>[2x]LLAGASSQRSVARMDGDVIIGALFSVHHQPPAEKVPERKCGEIREQYGIQRVEAMFHTLDKINADPVLLPNITLGSEIRDSCWHSSVALEQSIEFIRDSLISIRDEKDGINRCLPDGQSLPPGRTKKPIAGVIGPGSS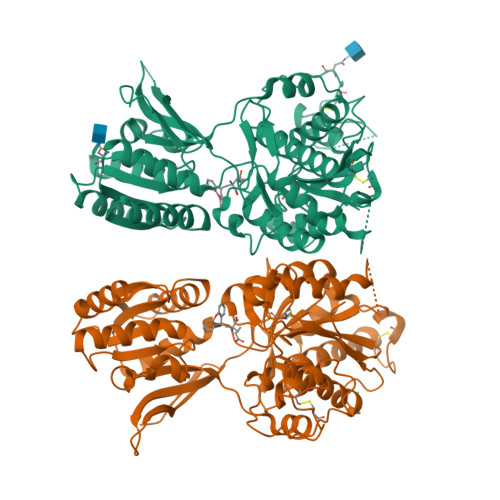SVAIQVQNLLQLFDIPQIAYSATSIDLSDKTLYKYFLRVVPSDTLQARAMLDIVKRYNWTYVSAVHTEGNYGESGMDAFKELAAQEGLSIAHSDKIYSNAGEKSFDRLLRKLRERLPKARVVVCFCEGMTVRGLLSAMRRLGVVGEFSLIGSDGWADRDEVIEGYEVEANGGITIKLQSPEVRSFDDYFLKLRLDTNTRNPWFPEFWQHRFQCRLPGHLLENPNFKRICTGNESLEENYVQDSKMGFVINAIYAMAHGLQNMHHALCPGHVGLCDAMKPIDGSKLLDFLIKSSFIGVSGEEVWFDEKGDAPGRYDIMNLQYTEANRYDYVHVGTWHEGVLNIDDYKIQMNKSGLVPRG2-{3-[3-(piperidin-4-yl)propoxy]phenyl}-N-[4-(pyridin-4-yl)-1,3-thiazol-2-yl]acetamide | C24 H28 N4 O2 S | 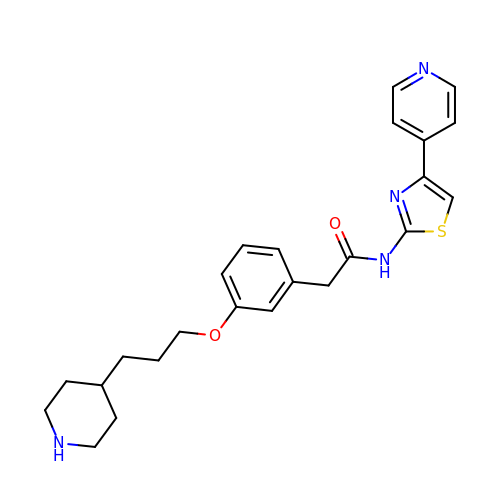IMDMAPNWXDTADU-UHFFFAOYSA-N>[11x]MSGRWSHPQFEKIHQRREAGARETCRDQIKGSDKDEEPSAALSHGQGYRPCGRPARNSKPEAGARPPAVPIMVNDPPVPALLWAQEVGHVLAGRARRLMLQFGVLFCTILLLLWVSVFLYGSFYYSYMP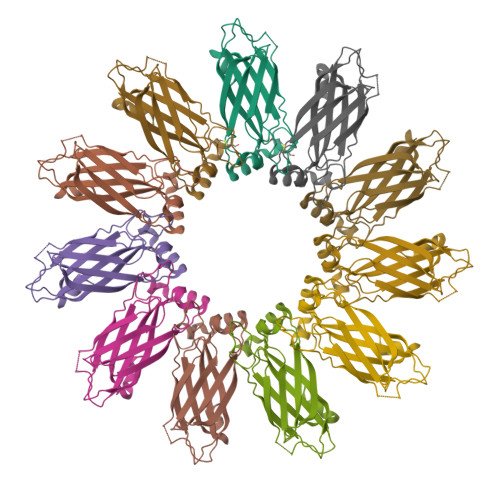TVSHLSPVHFHYRTDCDSSTASLCSFPVANVSLAKSGRDRVLMYGQPYRVTLELELPESPVNQDLGMFLVTVSCYTRGGRIISTSSRSVMLHYRSQLLQVLDTLLFSSLLLFGFAEQKQLLEVELYSDYRENSYVPTTGAIIEIHSKRIQMYGAYLRIHAHFTGLRYLLYNFPMTCAFVGVASNFTFLSVIVLFSYMQWVWGAVWPRHRFSLQVNIRQRDNSHHGAPRRISRHQPGQESTQQSDVTEDGESPEDPSGTEGQLSEEEKPEKRPLNGEEEQEPEASDGSWEDAALLTEANPPTSASASALAPETLGSLRQRPTCSSS> SMPTDIEDINPNVYDRIKERVLTANEEDENVPDPFDKREIFDLIRNINDPEHPLTLEELHVVQEDLIRINDSQNSVHISFTPTIPHCSMATLIGLSIRVKLLRSLPPRFKVTVEITPGTHASELAVNKQLADKERVAAALENNHLAEVINQCIAAKG;> SMGRLILEHTLQGHKGRIWGVAWHPKGNVFASCGEDKAIRIWSLTGNTWSTKTILSDGHKRTIREIRWSPCGQYLASASFDATTAIWSKSSGEFECNATLEGHENEVKSVSWSRSGGLLATCSRDKSVWIWEVAGDDEFECAAVLNPHTQDVKRVVWHPTKDILASASYDNTIKMFAEEPIDNDWDCTATLTSHTSTVWGIDFDADGERLVSCSDDTTIKIWRAYHPGNTAGVATPDQQTVWKCVC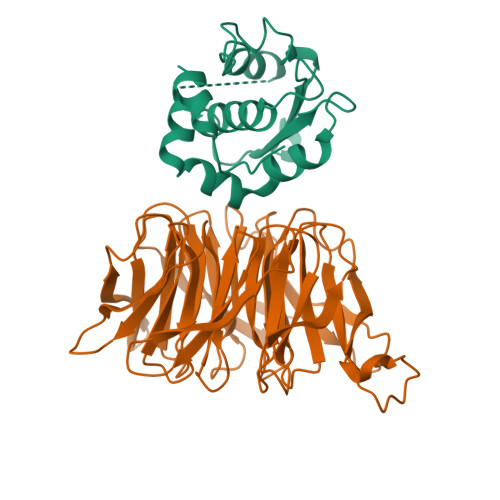TVSGQHSRAIYDVSWCKLTGLIATACGDDGIRIFKESSDSKPDEPTFEQITAEEGAHDQDVNSVQWNPVVAGQLISCSDDGTIKIWKVTE>GGIQGDLINEIDTFQNRIEIDPAHYRRGTDRPDLEGHCERIVSGSASIADAESTRENRKQKIVAECNNLRQALQELLTEYEKSTGRRDDNDDIPLGIAEVHKRTKDLRRHLRRAIVDHISDAFLDTRTPLILLIEAAKEGHEENTRYRSKMFQEHANEIVSVARLSCQLSSDVESVSVIQHTAAQLEKLAPQVAQAAILLCHQPTSKTAQENMETYKNAWFDKVRLLTTALDNITTLDDFLAVSEAHIVEDCERGIKGITANASTPDENAANCETVDCAAGSIRGRALRVCDVVDAEMDFLQNSEYTETVKQAVRILKTQRVDQFAERASALANRQEAHGLTWDPKTKEEEMNEFINACTLVHDAVK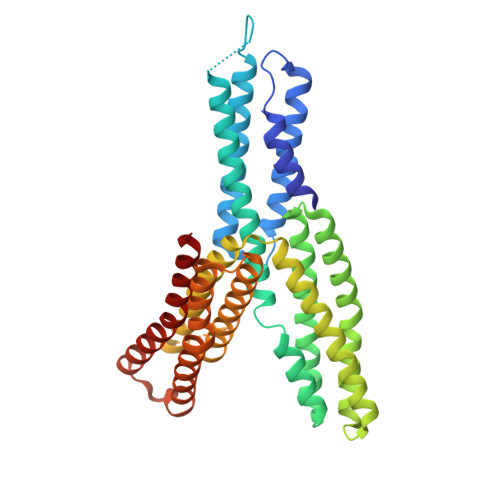DIRHALLMNRSMND[2x]5-methyl-1-[(3S)-1-{3-[3-(trifluoromethyl)phenoxy]benzyl}piperidin-3-yl]pyrimidine-2,4(1H,3H)-dione 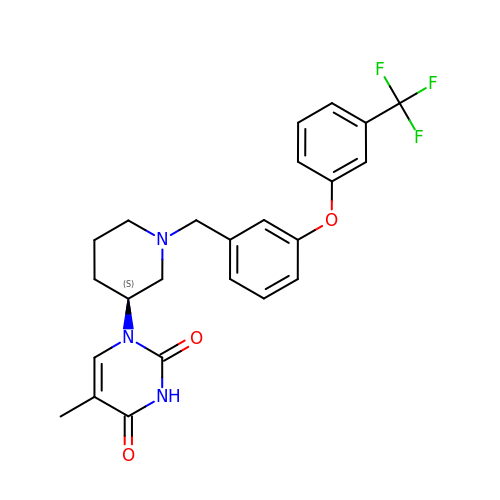| C24 H24 F3 N3 O3 | OVDFDRSJZJQKLN-IBGZPJMESA-N Here we describe the first crystal structure of an enzymatically active HD‐GYP phosphodiesterase protein, PmGH from Persephonella marina EX‐H1, a thermophilic marine member of the Aquificales. PmGH comprises an HD‐GYP domain fused to a GAF domain. A remarkable feature of the structure of PmGH was the identification of a trinuclear Fe centre which is buried at the bottom of the cavity forming the c‐di‐GMP binding site.

Structures of complexes of PmGH with GMP and c‐di‐GMP were determined from crystal soaking experiments with both nucleotides. Crystal soaks with GMP and c‐di‐GMP gave identical structures of PmGH in complex with GMP showing that PmGH retained phosphodiesterase activity in the crystal. Based on the structure of the complex of PmGH with the final reaction product GMP, which shows the 5′‐phosphate of GMP bound to the M‐H Fe pair, c‐di‐GMP hydrolysis may be catalysed by these two sites alone, with the G‐site Fe contributing to the hydrolysis rate. This would invoke primarily a two‐metal‐ion mechanism as seen for other PDEs (Barends et al., 2009; Tchigvintsev et al., 2010). In this case, the two scissile c‐di‐GMP phosphates would be sequentially hydrolysed by the M‐H Fe pair with the phosphate group which initially binds to the hydroxyl group of Y285 being brought into a similar conformation to the phosphate group bound to the M‐site Fe(III). After hydrolysis of this M‐site bound phosphate group, the hydrolysable phosphate group of 5′‐phosphoguanylyl‐(3′‐5′)‐guanosine (5′‐pGpG), the product of this first hydrolysis step, can be positioned in a similar conformation to the previously hydrolysed phosphate by a rotation around the original twofold axis of the intact c‐di‐GMP. This would then enable the conversion of the now bound 5′‐pGpG to GMP.

>[2x]GPGYQDPERKLKILLDYSSKIANEKDLRNVLLFLTDLAKEIMEADRASIFLYDDQKKTLWTIVAHGVDRIEIDADKGIAGYVFRTGEILNIPDAYKDPRFDRDIDKRTGYRTRTILAVPLFDRKQNIIGVFQVINKLTNSVFTEEDIELLRHISLYASSTIENAILYEKLKKAHEDVIYRLSHATKFKDPETQNHIIRVGLYAEILAREAGLDEEDVELVKLAAPMHDIGKVGIPDRVLLKPGKLNDEEWEIMKKHTIYGYEILKGGDSRLLQIAADIAIEHHERWDGTGYPFGKKGEEISIYGRMTSISDVFDALTSDRPYKKAWDMDRTVRFFKEQKGKHFDPFLTDIFLKNIDQMFSIKRELRDED>SNAIKTTATLFLHGYGGSERSETFMVKQALNKNVTNEVITARVSSEGKVYFDKKLSEDAANPIVKVEFKDNKNGNFKENAYWIKEVLSQLKSQFGIQQFNFVGHSMGNMSFAFYMKNYGDDRHLPQLKKEVNIAGVYNGILNMNENVNEIIVDKQGKPSRMNAAYRQLLSLYKIYCGKEIEVLNIYGDLEDGSHSDG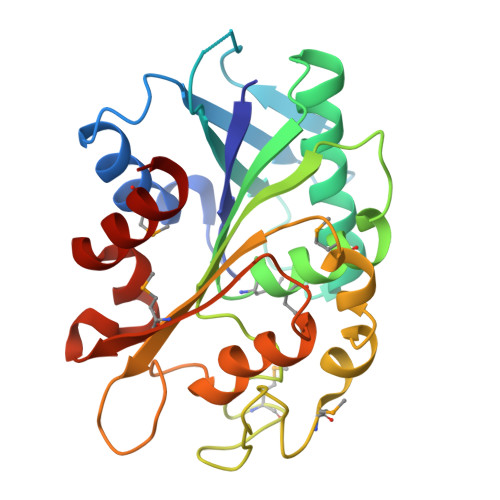RVSNSSSQSLQYLLRGSTKSYQEMKFKGAKAQHSQLHENKDVANEIIQFLWE[2x]> SSVFVPDEWEVSR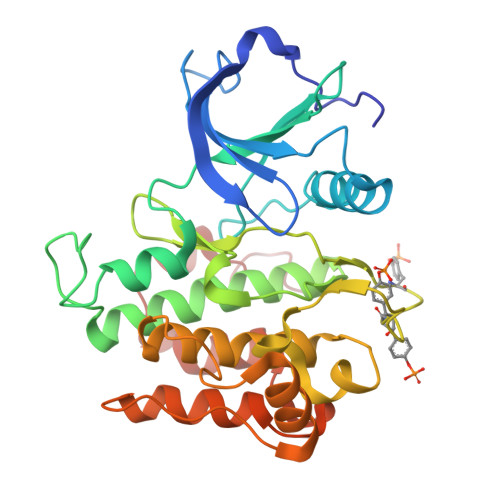EKITLLRELGQGSFGMVYEGNARDIIKGEAETRVAVKTVNESASLRERIEFLNEASVMKGFTCHHVVRLLGVVSKGQPTLVVMELMAHGDLKSYLRSLRPEAENNPGRPPPTLQEMIQMAAEIADGMAYLNAKKFVHRDLAARNCMVAHDFTVKIGDFGMTRDIYETDYYRKGGKGLLPVRWMAPESLKDGVFTTSSDMWSFGVVLWEITSLAEQPYQGLSNEQVLKFVMDGGYLDQPDNCPERVTDLMRMCWQFNPKMRPTFLEIVNLLKDDLHPSFPEVSFFHSEENK2-(7-AMINO-6-METHYL-3H-PYRAZOLO[4,3-D]PYRIMIDIN-3-YL)-5-HYDROXYMETHYL-TETRAHYDRO-FURAN-3,4-DIOL 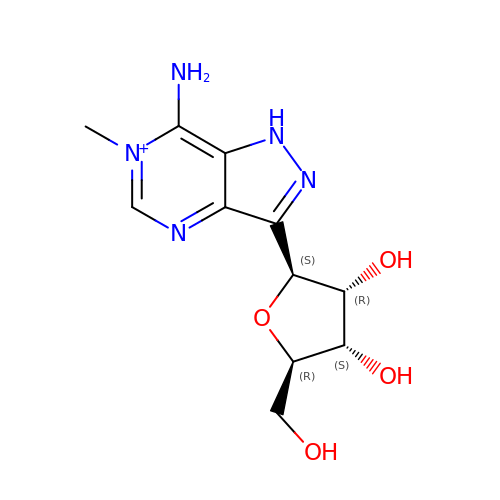| C11 H16 N5 O4 | UHYKIYIKTWEXSX-LFAOKBQASA-O>TEAQKCNLQGQWRNKLGSNLIIESVSQNGEFTGTYFTSVSLTNSTIRISPLTGYQKLTEKPTFGFTVHWAFSDSITVWTGQCFLNEKGEEILHTMWLLRSSQEKEQDNWTGTRVGANTFTRLSKKKIRKE[2x]

Here we report, to our knowledge, the first biochemical and structural characterization of an amphibian avidin - xenavidin - a frog avidin from Xenopus tropicalis. In general, both of the xenavidin structures were highly similar to the known structures of avidin and streptavidin: the 3D structure of xenavidin is homotetrameric, each subunit consisting of an eight-stranded β-barrel. The amino acids lining the biotin-binding pocket are structurally conserved between xenavidin and chicken avidin. Our results show that xenavidin is a well-conserved member of the avidin protein family having a tetrameric structure, N-glycosylation and extremely tight biotin-binding capability that is mediated via numerous non-covalent interactions including hydrogen bonds, hydrophobic interactions and van der Waals contacts.

Xenavidin overexpressed in insect cells was crystallized with and without D-biotin (BTN) added to the crystallization solution. The structures crystallized in a rhombohedral space group and had a dimer in their asymmetric unit (for the structure determination statistics). The subunits of the dimer found in the asymmetric units of the xenavidin crystals are labelled A and D to match the numbering system generally used to describe the biological unit of chicken avidin (tetramer; subunits I-IV;). In the unliganded structure of xenavidin, there was no clear electron density for biotin in subunit A. However, weak electron density was evident for the ligand at the binding site in subunit D; thus, a biotin molecule was built into subunit D of the unliganded xenavidin structure despite the presence of weak electron density around the ligand. In the BTN-complex structure, D-biotin was clearly present in both of the biotin-binding sites of the asymmetric unit. A water molecule was detected in the unliganded structure of xenavidin at the bottom of the ligand-binding site bridging the carboxamide group of N117 and biotin (bridging was evident only in subunit D); the conformation of N117 in the unliganded structure differs from that in the structure of the xenavidin-biotin complex. Thus, the unliganded structure of xenavidin may represent the first example of an intermediate structure of the avidin family, with a structural water molecule located deep within the biotin-binding pocket and lending support to the water-bridged model of biotin association/dissociation. Interestingly, N117, the residue analogous to D128 of streptavidin and N118 of avidin, has an altered conformation in unliganded xenavidin compared to N117 of the biotin-complex structure of xenavidin, suggesting a potentially important role for this residue in the water-mediated association/dissociation mechanism of avidins in general.> EPYTDSNVPEGDSVPEAHWTKLQHSLDTALAAARSAPTAPIAARVTGQTRNITVDPRLFKAARLHSPRVLFSTQPPPTSSDTLDLDFQAHGTIPFNRTHRSAASSTHPVFHMGEFSVCDSVSVWVGDKTTATDIKGKEVTVLAEVNINNSVFRQYFFETKCRASNPVESGCRGIDSKHWNSYCTTTHTFVKALTTDEKQAAWRFIRID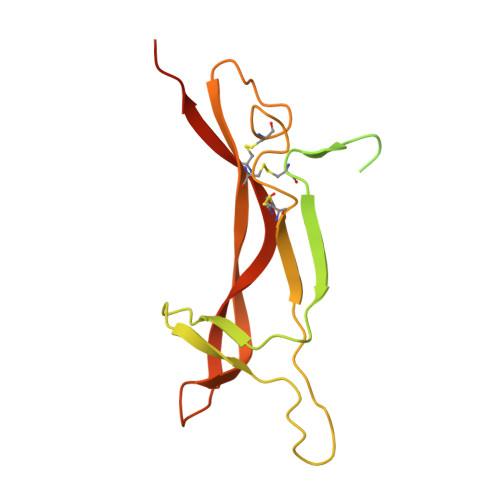TACVCVLSRKATAAGHHHHHHH> TPAFNKPKVELHVHLDGAIKPETILYFGKKRGIALPADTVEELRNIIGMDKPLSLPGFLAKFDYYMPVIAGCREAIKRIAYEFVE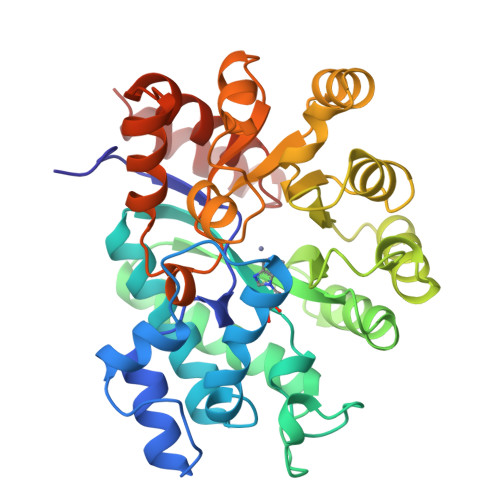MKAKEGVVYVEVRYSPHLLANSKVDPMPWNQTEGDVTPDDVVDLVNQGLQEGEQAFGIKVRSILCCMRHQPSWSLEVLELCKKYNQKTVVAMDLAGDETIEGSSLFPGHVEAYEGAVKNGIHRTVHAGEVGSPEVVREAVDILKTERVGEGYHTIEDEALYNRLLKENMHFEVCPWSSYLTGAWDPKTTHAVVRFKNDKANYSLNTDDPLIFKSTLDTDYQMTKKDMGFTEEEFKRLNINAAKSSFLPEEEKKELLERLYREYQ> SNASEPVTIVLSQMGWVRSAKGHDIDAPGLNYKAGDSFKAAVKGKSNQPVVFVDSTGRSYAIDPITLPSARGQGEPLTGKLTLPPGATVDHMLMESDDQKLLMASDAGYGFVCTFNDL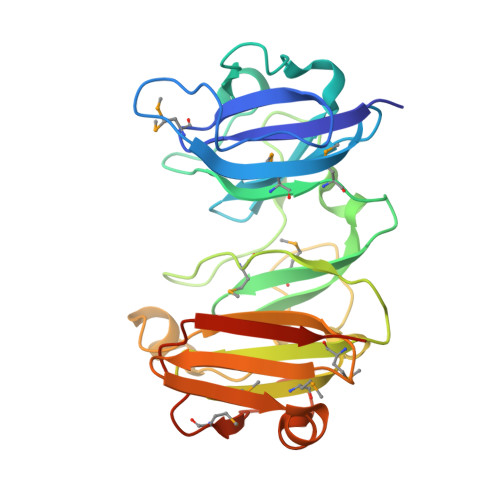VARNRAGKALITLPENAHVMPPVVIEDASDMLLAITQAGRMLMFPVSDLPQLSKGKGNKIINIPSAEAARGEDGLAQLYVLPPQSTLTIHVGKRKIKLRPEELQKVTGERGRRGTLMRGLQRIDRVEIDSPRRASSGDSEE> MANELTWHDVLAEEKQQPYFLNTLQTVASERQSGVTIYPPQKDVFNAFRFTELGDVKVVILGQDPYHGPGQAHGLAFSVRPGIAIPPSLLNMYKELENTIPGFTRPNHGYLESWARQGVLLLNTVLTVRAGQAHSHASLGWETFTDKVISLINQHREGVVFLLWGSHAQKKGAIIDKQRHHVLK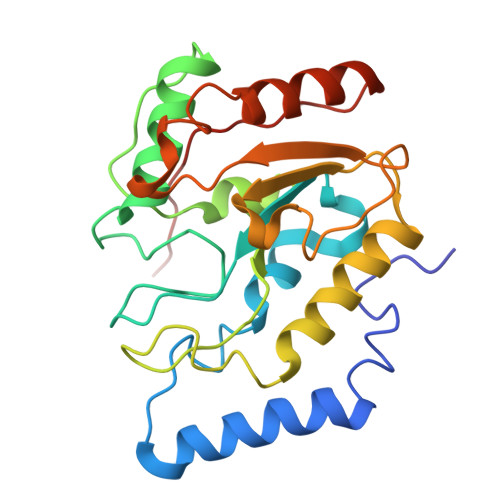APHPSPLSAHRGFFGCNHFVLANQWLEQRGETPIDWMPVLPAESE>[2x]MEMRVLLIAGGVSPEHEVSLLSAEGVLRHIPFPTDLAVIAQDGRWLLGEKALTALEAKAAPEGEHPFPPPLSWERYDVVFPLLHGRFGEDGTVQGFLELLGKPYVGAGVAASALCMDKDLSKRVLAQAGVPVVPWVAVRKGEPPVVPFDPPFFVKPAN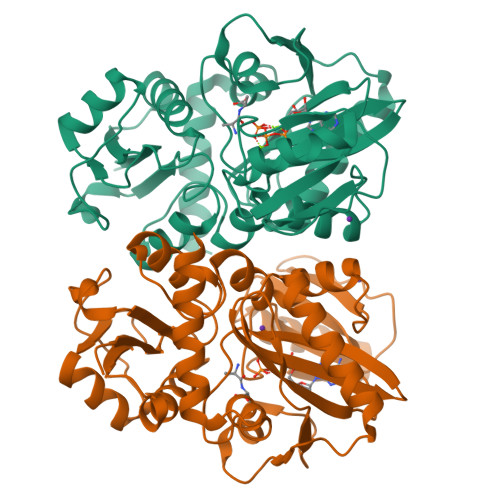TGSSVGISRVERFQDLEAALALAFRYDEKAVVEKALSPVRELEVGVLGNVFGEASPVGEVRYEAPFYDYETKYTPGRAELLIPAPLDPGTQETVQELALKAYKVLGVRGMARVDFFLAEGELYLNELNTIPGFTPTSMYPRLFEAGGVAYPELLRRLVELALTHHHHHH Cotton bollworm (Helicoverpa armigera) is a worldwide agricultural pest in which the transport of pheromones is indispensable and perceived by pheromone-binding proteins (PBPs). Here, we solved three structures of the cotton bollworm HarmPBP1 at different pH values and its complex with ligand, Z-9-hexadecenal. The HarmPBP1 scaffold contains three conserved disulfide bonds linking α-helices α1 and α3 (Cys46-Cys81), α3 and α6 (Cys77-Cys136), and α5 and α6 (Cys124-Cys145), encapsulating the hydrophobic pocket for pheromones binding. The structure of HarmPBP1 was found to contain a hydrophobic cavity formed by the five helices α1, α3, α4, α5, and α6.

The apo-HarmPBP1 structure at pH 7.5 was determined by molecular replacement and refined to a resolution of 1.3 Å in the space group of P21, with an Rwork of 17.9% and an Rfree of 19.8%. The structure was built in the electron density map, except for the C-terminal residues 159-170. Although apo-HarmPBP1 adopts a common PBP scaffold of six α-helices surrounding a predominantly hydrophobic central pocket, the conformation is greatly distinct from other apo-PBPs. Surprisingly, the structural similarity between apo-HarmPBP1 and all other apo-GOBPs or apo-PBPs was lower as the RMSD was larger than 1.5 Å, revealing a distinct conformation of apo-HarmPBP1 compared with other apo-PBPs. The most significant structural differences between apo-HarmPBP1 and other known insect PBPs were observed at the C terminus. The last 12 residues were missed in the structure of apo-HarmPBP1, which might have been a result of crystal packing. However, the conformations of both termini as well as some loops differed significantly between apo-HarmPBP1 and the apo-BmorPBP/apo-ApolPBP1. The first helix of HarmPBP1 occupied the C-terminal helix position of the above two structures. In the apo-HarmPBP1, there was a channel through the ligand binding pocket. In the apo-HarmPBP1 structure, part of the Lys138 side chain was flexible. Moreover, the arrangements of both proteins in the crystal packing were different, revealing that the little structural difference was not caused by experimental errors.

> GSMASQDVIKNLSMNFAKPLEDCKKEMDLPDSVTTDFYNFWKEGYEFTNRQTGCAILCLSSKLELLDQELKLHHGKAQEFAKKHGADDAMAKQLVDLIHGCAQSTPDVADDPCMKTLNVAKCFKAKIHELNWAPSMELVVGEVLAEV>MVKDEIVISSALRTPIGAFSGTLKDTPAAALGAHVVKTLLERTGLAPERVDEVVMGNVLQAGNGMNVARQVAVNGGLPVAVPAHTVNRVCGSGAQAVVTAYAQ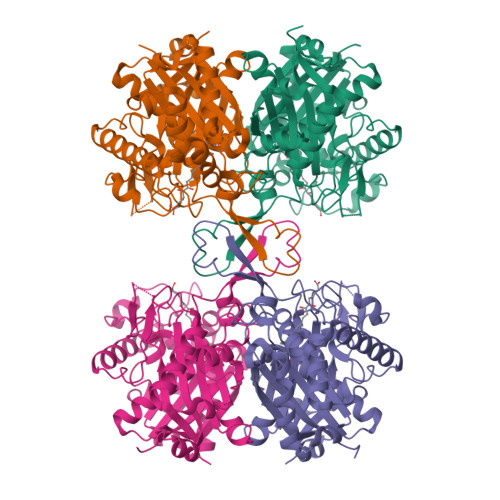IRSGLSNLVIAGGVENMDQAPYLMPSLRHGARMGHTQALDALLRDGLNDAFSDQHSGWHTEDLVAKYEVSREAQDRFAATSQQRFAAAQAAGWFEGEIVPVTITTRKGETVFAKDEANRPDTTEAGLAKLRPAFRKDGTITAGNAPGLNAGAAAMIVSSHATATELGLQPQLVIRGIGVAAVEPGLFGFGPVPAIKLALAQAQWQVQDVDRFEVNEAFAAVGLVVRDELGIAPERFNVDGGAIAHGHPIGATGAILLTKVAHALRRTSERRAVVSLCIGGGQGIALALERVKLAAALEHHHHHH[4x]2-AMINO-6-(2-PHENYLETHYL)PYRIMIDIN-4(3H)-ONE | C12 H13 N3 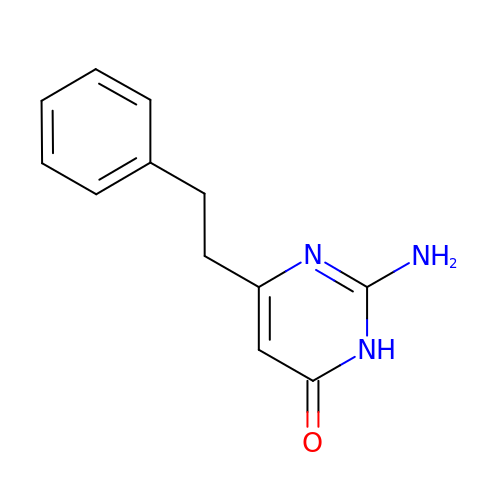O | CNBSPUGFNQVSJS-UHFFFAOYSA-N>MAEIPKEMLRAQTNVILLNVLKQGDNYVYGIIKQVKEASNGEMELNEATLYTIFKRLEKDGIISSYWGDESQGGRRKYYRLTEIGHENMRLAFESWSRVDKIIENLEANKKSEAIKHHHHHH[2x]

LmrR is a transcriptional repressor regulating the expression of the multidrug ABC transporter LmrCD. In the apo state, LmrR shows high affinity for the promotor region of LmrRCD. This affinity is reduced upon binding of a drug at its drug-binding site, enabling expression of the multidrug transporter. LmrR is a homodimeric protein with the drug binding site at the dimer interface.19 Central in this binding site are two Trp residues, W96 and W96′ (residue 96 from the other monomer), oriented face-to-face at 7 Å from each other.

To investigate the importance of π–π interactions for drug binding, the electron density in the π electron cloud of W96 was modulated by progressive fluorination of the W96 indole side chain. To assess whether the Trp analogs influence the overall structure of LmrR and its drug-binding pocket, crystal structures were determined of LmrR with bound Dau for LmrR variants 5FW, 5,6diFW, and 5,6,7triFW. The crystal structures belong to the same crystal form (space group C2 with very similar unit cell dimensions) and were refined to resolutions varying between 2.55 and 2.15 Å. Although the crystal structures show generally good geometry, they all suffer from high crystallographic B-factors (average B-factors for protein atoms varying between ∼57 and ∼89 Å2), indicative of static disorder in the crystals. Nevertheless, the electron density maps were of sufficient quality to identify the Trp analogs at positions 67 and 96 in both polypeptide chains of the dimeric LmrR variants. No major differences were observed in the backbone and side chain conformations around residues W67 and W96, compared to wild-type LmrR.19 Moreover, as shown in Figures 2 and S6, the binding mode of Dau to LmrR is not substantially affected by the presence of the fluorinated Trp analogs. Dau is bound in the same way as in the wild-type protein, with the aromatic part of Dau sandwiched between two Trp analog residues, stabilized by π–π stacking interactions. Thus, we conclude that the different Dau binding affinities observed for the LmrR variants are not related to conformational changes of the protein or significantly altered ligand binding modes. The binding affinities of LmrR for Dau and RBF decreased upon increasing degrees of fluorination of W96. Dau behaved less extreme, with the kd decreasing 6-fold.>MPRKIILDCDPGIDDAVAIFLAHGNPEIELLAITTVVGNQSLEKVTQNARLVADVAGIVGVPVAAGCTKPLVRGVRNASHIHGETGMGNVSYPPEFKTKLDGRHAVQLIIDLIMSHEPKTITLVPTGGLT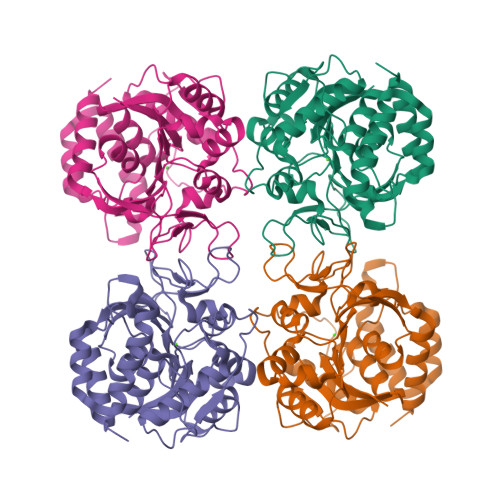NIAMAVRLEPRIVDRVKEVVLMGGGYHTGNASPVAEFNVFIDPEAAHIVFNESWNVTMVGLDLTHLALATPAVQKRVREVGTKPAAFMLQILDFYTKVYEKEHDTYGKVHDPCAVAYVIDPTVMTTERVPVDIELNGALTTGMTVADFRYPRPKNCRTQVAVKLDFDKFWCLVIDALERIGDPQ[4x]>MGSSHHHHHHSSGRENLYFQGQHLLKNPGILDKIIYAAKIKSSDI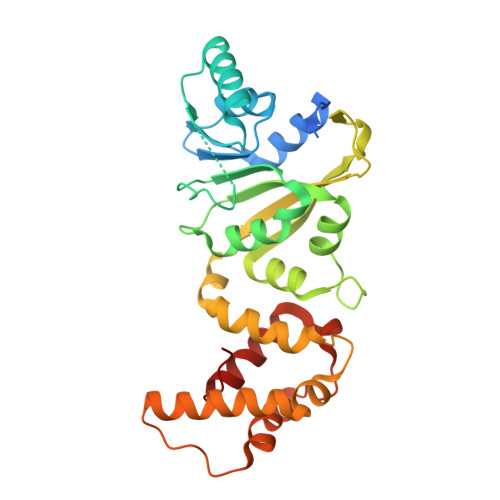VLEIGCGTGNLTVKLLPLAKKVITIDIDSRMISEVKKRCLYEGYNNLEVYEGDAIKTVFPKFDVCTANIPYKISSPLIFKLISHRPLFKCAVLMFQKEFAERMLANVGDSNYSRLTINVKLFCKVTKVCNVNRSSFNPPPKVDSVIVKLIPKESSFLTNFDEWDNLLRICFSRKRKTLHAIFKRNAVLNMLEHNYKNWCTLNKQVPVNFPFKKYCLDVLEHLDMCEKRSINLDENDFLKLLLEFNKKGIHFFNI[2x]>MNYGITESVKTTRSKIKIKDIVSDVVEKKANAIKYFLEGEEFKQAIVFGAYLSGSYIAYSLLKDCEEVIIVDIQPHLKDILFNDGIKFMDLNKLQLELRNGTSINPDLVIDLTGIGGVSPDLISKFNPKVLIVEDPKGNHDKGISKIDNTDKRLCVGAKKGVLKTYRSSKFSKTSGTMTLVVDIIMDSCREINELDSVLYTIPNLKYFEGTVFHEKNVKKFLTELNMSAITVSSIDHVEYELEEILSKNISRVDSFVKEFDKLAAALEHHHHHH[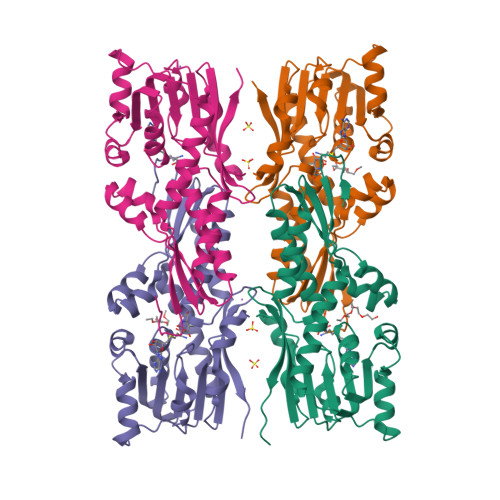4x]> GPKEVYLDRKLLTLEDKE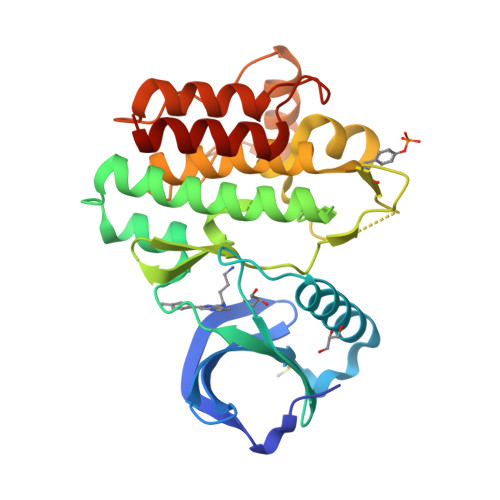LGSGNFGTVKKGYYQMKKVVKTVAVKILKNEANDPALKDELLAEANVMQQLDNPYIVRMIGICEAESWMLVMEMAELGPLNKYLQQNRHVKDKNIIELVHQVSMGMKYLEESNFVHRDLAARNVLLVTQHYAKISDFGLSKALRADENYYKAQTHGKWPVKWYAPECINYYKFSSKSDVWSFGVLMWEAFSYGQKPYRGMKGSEVTAMLEKGERMGCPAGCPREMYDLMNLCWTYDVENRPGFAAVELRLRNYYYDVVN> MAGWQSYVDNLMCDGCCQEAAIVGYCDAKYVWAATAGGVFQSITPVEIDMIVGKDREGFFTNGLTLGAKKCSVIRDSLYVDGDCTMDIRTKSQGGEPTYNVAVGRAGRVLVFV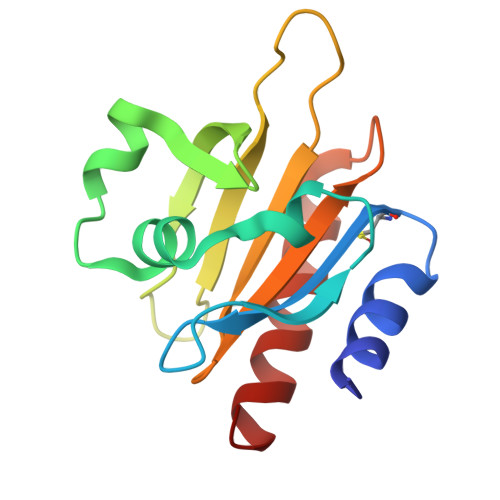MGKEGVHGGGLNKKAYSMAKYLRDSGF>[60x]MWRVCARRAQNAAPRAGFGARWTALREEPGAPCAAPRAGSVPARCSSTTRGYGRSRALCGWSASSWATPQNRILLQLWGSPNRRWYSLPPHQKVPLPSLSPTMQAGTIARWEKKEGDKINEGELIAEVETDKATVGFESLEECYMAKILVAEGTRDVPVGAIICITVEKPEDIEAFKNYTLDSSAAPAPQAAPAPTPAAAAPAPTPSAQAPGSSYPTHMQVVLPALSPTMTMGTVQRWEKKVGEKLSEGDLLAEIETDKATIGFEVQEEGYLAKILIPEGTRDVPLGTPLCIIVEKEADIPAFADYRPTEVTDLKPPAPPPTPSPVTPVPPAPQPVAPTPAATRPATPAGPKGRLFVSPLAKKLASEKGIDLTQIKGTGPDGRIIKKDIDSFVPTKAAPPPA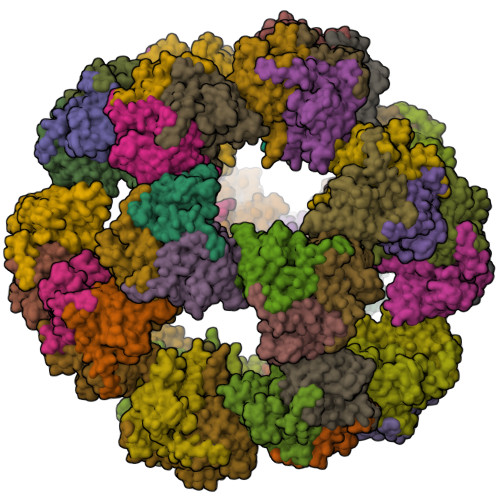AAVPPPSPGVAPVPTGVFTDIPISNIRRVIAQRLMQSKQTIPHYYLSVDVNMGEVLLVRKELNKMLEGRSKISVNDFIIKASALACLKVPEANSSWLDTVIRQNHVVDISVAVSTPAGLITPIVFNAHIKGLETIANDVVSLATKAREGKLQPHEFQGGTFTISNLGMFGIKNFSAIINPPQACILAVGASEDRLFPADNEKGFDVASMMSVTLSCDHRVVDGAVGAQWLAEFRKYLEKPITMLL> MSLMGYKNNRVGYQKELLTSRAVIKKDNYAIIPHDGLVQNAVPGFENVDISILGSPKLGATFVDYIATFHKNGQQTTGFGGDGIQTLVYVIDGRLRVSDGQETHE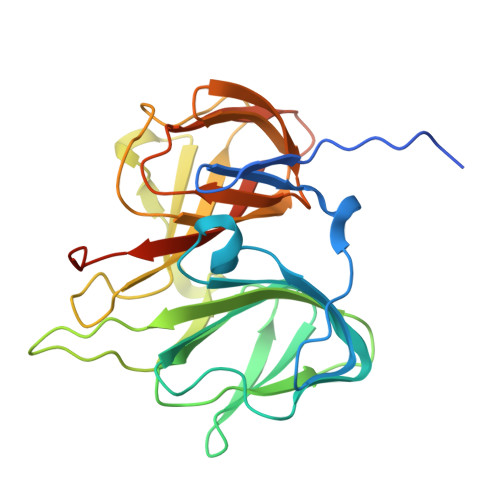LEAGGYAYFTPEMKMYLANAQEADTEVFLYKKRYQPLAGHQPYKVVGSIHDQQPEEYEGMTDVLLWSLLPKEFDFDMNMHILSFEPGASHAYIETHVQEHGAYLISGQGMYNLDNEWYPVEKGDYIFMSAYVPQAAYAVGREEPLMYVYSKDANREPELEGGSHHHHHH((2R,3S,4R,5R)-5-(6-AMINO-9H-PURIN-9-YL)-3,4-DIHYDROXY-TETRAHYDROFURAN-2-YL)METHYL 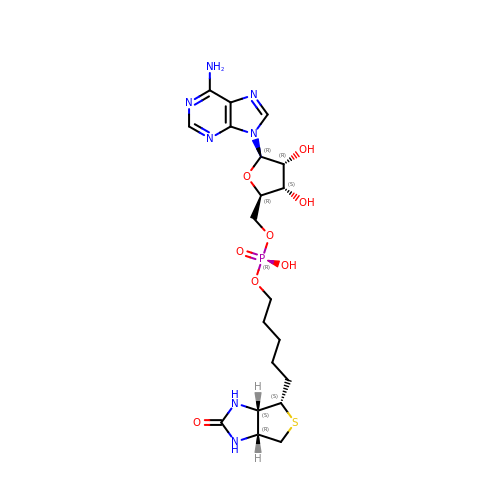5-((3AS,4S,6AR)-2-OXO-HEXAHYDRO-1H-THIENO[3,4-D]IMIDAZOL-4-YL)PENTYL HYDROGEN PHOSPHATE | C20 H30 N7 O8 P S | KBOGUFFJCBPJEH-SQGSUPJISA-N>[4x]EQTAAPAKPVTVEAKNETFAPQHPDQYLSWKATSEQSERVDALAEDPRLVILWAGYPFSRDYNKPRGHAFAVTDVRETLRTGAPKNAEDGPLPMACWSCKSPDVARLIQKDGEDGYFHGKWARGGPEIVNNLGCADCHNTASPEFAKGKPELTLSRPYAARAMEAIGKPFEKAGRFDQQSMVCGQCHVEYYFDGKNKAVKFPWDDGMKVENMEQYYDKIAFSDWTNSLS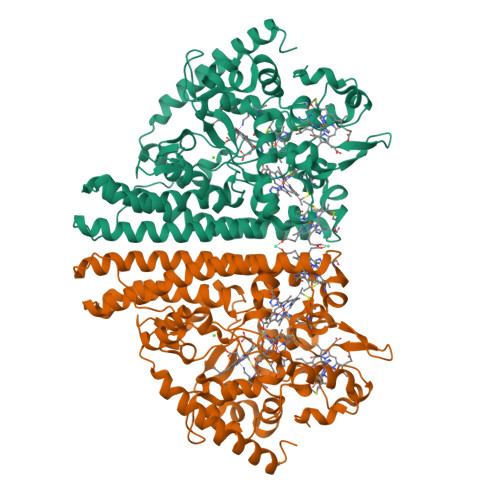KTPMLKAQHPEYETWTAGIHGKNNVTCIDCHMPKVQNAEGKLYTDHKIGNPFDNFAQTCANCHTQDKAALQKVVAERKQSINDLKIKVEDQLVHAHFEAKAALDAGATEAEMKPIQDDIRHAQWRWDLAIASHGIHMHAPEEGLRMLGTAMDKAADARTKLARLLATKGITHEIQIPDISTKEKAQQAIGLNMEQIKAEKQDFIKTVIPQWEEQARKNGLLSQ>GPLGSPEFMASGGGGCSASERLPPPFPGMDPESEGAAGGSEPEAGDSDTEGEDIFTGAAAATKPQSPKKTTSLFPIKNGSKENGIHEDQDQEPQDLFADATVELSLDSTQNNQKTMPGKTLTSHPPQEATNSPKPQPSYEELEEEQEDQFDLTVGITDPEKIGDGMNAYVAYKVTTQTSLPMFRSRQFAVKRRFSDFLGLYEKLSEKHSQNGFIVPPPPEKSLIGMTKVKVGKEDSSSAEFLEKRRAALERYLQRIVNHPTMLQDPDVREFLEKEELPRAVGTQALSGAGLLKMFNKATDAVSKMTIKMNESDIWFEEKLQEVECEEQRLRKLHAVVETLVNHRKELALNTALFAKSLAMLGSSEDNTALSRALSQLAEVEEKIEQLHQEQANNDFFLLAELLSDYIRLLAIVRAAFDQRMKTWQRWQDAQATLQKKRESEARLLWANKPDKLQQAKDEITE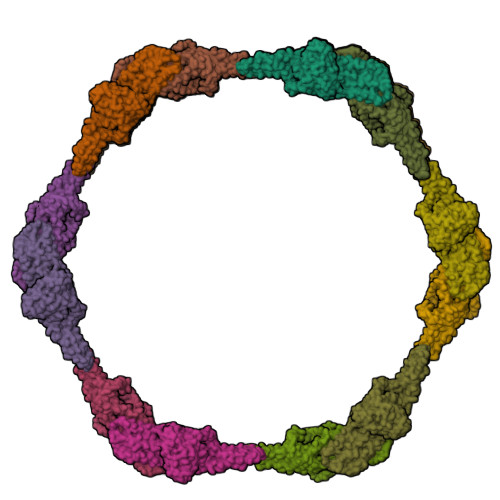WESRVTQYERDFERISTVVRKEVTRFEKEKSKDFKNHVMKYLETLLHSQQQLAKYWEAFLPEAKAIS[16x]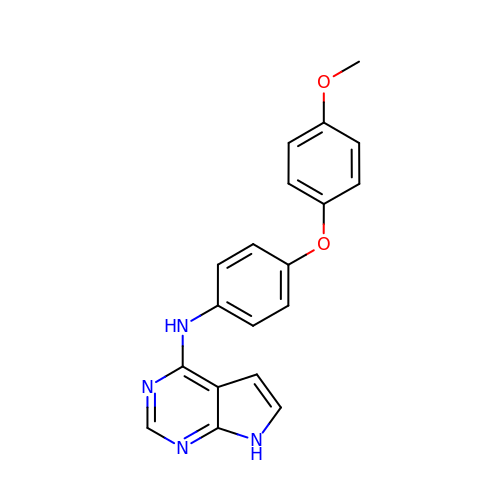~{N}-[4-(4-methoxyphenoxy)phenyl]-7~{H}-pyrrolo[2,3-d]pyrimidin-4-amine | C19 H16 N4 O2 | BDYNACMDWPBSRV-UHFFFAOYSA-N>[3x]MAHHHHHHMQFNDILAALDIDLAQWKGNALTARSPLDGATLATLAVDTPADAERKIDAAHDAFLKWRTVPAPVRGELVRVFGNVLREHKAELGRLVTLEAGKITSEGLGEVQEMIDICDFAVGLSRQLYGLTIASERPGHRMMETWHPIGVCGVISAFNFPVAVWAWNAALAFVCGDSVVWKPSEKTPLTAIACHVLLQKALREFEKTHPGVAPAELGQLVLGMRDVGEVLTASKKVPVVSATGSVRMGQEVAKVLSQRLARGILELGGNNGMIVAPSADLDLVVRAVTFAAVGTAGQRCTTLRRLIVHRSLVEQLLPRIEKAYASVKVGNPLEEGTLVGPLVDRASFDAMQKALADAREQGGEVKGGERVDVGHADAYYVRPAIVRMPKQSAVVERETFAPILYVMVYDNFDDAIDVHNAVPQGLSSAIFTNDMREAEQFMSAAGSDCGIVNVNIGTSGAEIGGAFGGEKETGGGRESGSDAWKAYMRRATNTINYSRQLP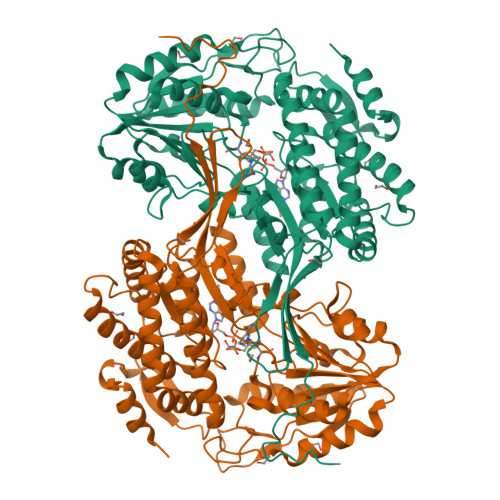LAQGVKFDV> GMSKPAITLWSDAHFFSPYVLSAWVALQEKGLSFHIKTIDLDSGEHLQPTWQGYGQTRRVPLLQIDDFELSESSAIAEYLEDRFAPPTWERIYPLDLENRARARQIQAWLRSDL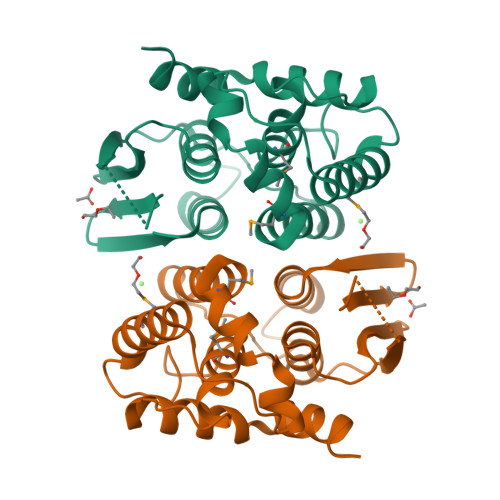MPIREERPTDVVFAGAKKAPLTAEGKASAEKLFAMAEHLLVLGQPNLFGEWCIADTDLALMINRLVLHGDEVPERLVDYATFQWQRASVQRFIALSAKQSG N~5~-[2-(ethylsulfanyl)ethanimidoyl]-L-ornithine | C9 H19 N3 O2 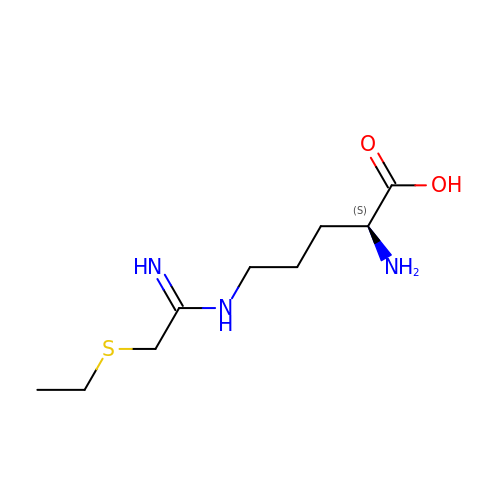S | GKZCWWBQARDOFD-ZETCQYMHSA-N>[4x]DPDPSQLHRSSLVKNLQNIYFLYEGDPVTHENVKSVDQLLSHDLIYNVSGPNYDKLKTELKNQEMATLFKDKNVDIYGVEYYHLCYLCENAERSACIYGGVTNHAGN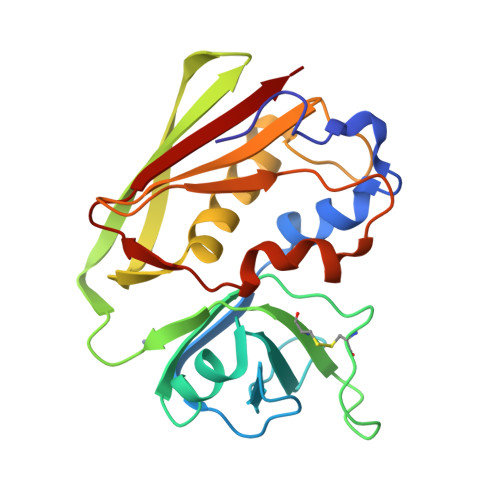HLEIPKKIVVKVSIDGIQSLSFDIETNKKMVTAQELDYKVRKYLTDNKQLYTNGPSKYETGYIKFIPKNKESFWFDFFPEPEFTQSKYLMIYKDNETLDSNTSQIEVYLTT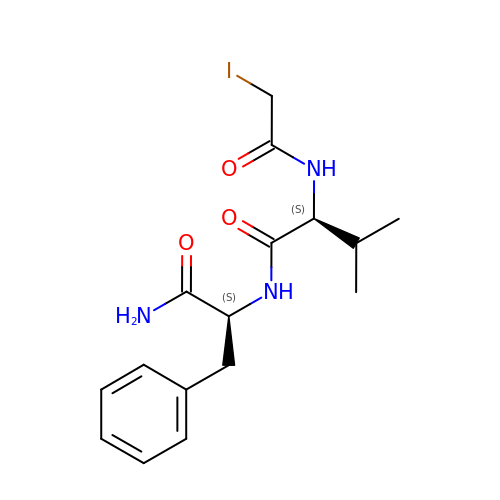N-(iodoacetyl)-L-valyl-L-phenylalaninamide | C16 H22 I N3 O3 | IBXSBHDYMGMZJA-JSGCOSHPSA-N> GPLGSRGGRGGGD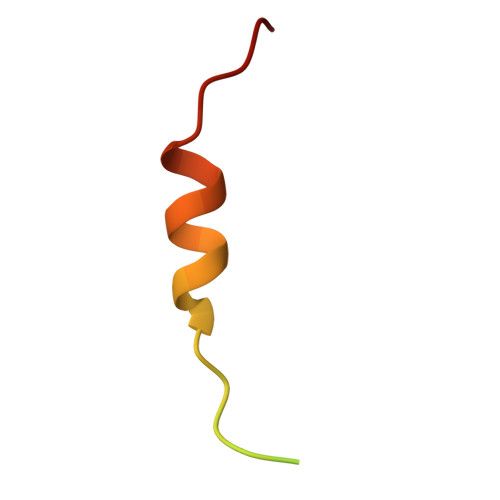RGGFGPGKMDSRGEHRQDRRERPY> MAKSHHHHHHTSVENNALSLVARGCAVAAPCRTKVAEQLLEIGAKAGMAG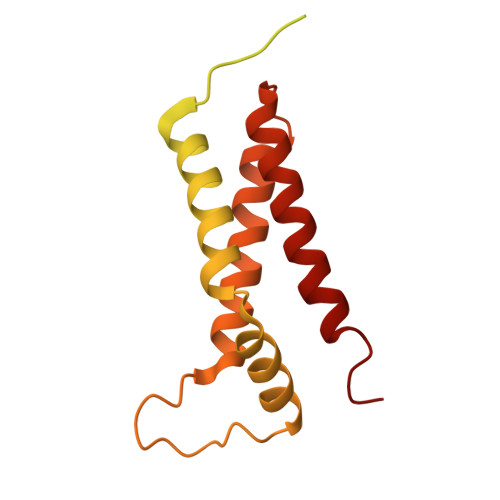LAGAAVKDMADRMTSDELEHLITLQMMGNDEITTKYLSSLHDKYGSGAASNPNIGKDLTDAEKVELGGSGSGTGTPPPSENDPKQQNEKTVDKLNQKQESAIKKIDNTIKNALKDHDIIGTLKDMDGKPVPKENGGYWDAMQEMQNTLRGLRNHADTLKNVNNPEAQAAYGRATDAINKIESALKGYGI>[2x]GPGTSRQCQEQLKEVNKTCEALLFKLGEKVKTLEME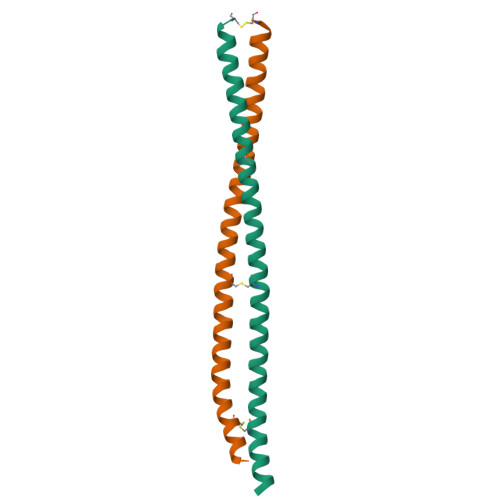VAKEKAVCSKDKESLLAGKRQTEEQLEACGKARERQQQEQQVTEENLRKVQSLCIPLDQ> DCPSGWSSYEGHCYKPFKLYKTWDDAERFCTEQAKGGHLVSIESAGEADFVAQLVTENIQNTKSYVWIGLRVQGKEKQCSSEWSDGSSVSYENWIEAESKTCLGLEKETGFRKWVNIYCGQQNPFVCEA;> DCPSDWSSYEGHCYKPFSEPKNWADAENFCTQQHAGGHLVSFQSSEEADFVVKLAFQTFGHSIFWMGLSNVWNQCNWQWSNA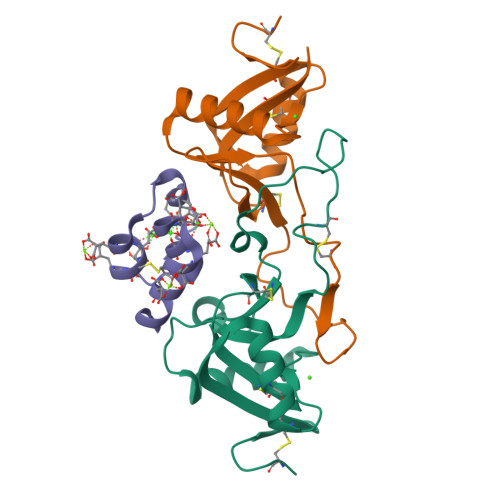AMLRYKAWAEESYCVYFKSTNNKWRSRACRMMAQFVCEFQA;> YNSGKLEEFVRGNLERECKEEKCSFEEAREVFENTEKTTEFWKQYV> MNLEVLCGRINVENGLSLGEPGLYDQIYDRPGLPDLDVTVDATGVTVDIGAVPDSASQLGSSINAGLITIQLSEAYKINHDFTFSGLSKTTDRRLSEVFPITHDGSDGMTPAVIHTRLDGTIVVVEFSTTRSHNIGGLEAAYRTKIEKYRDPISRRVDIMENPRVFFGVIVVSSGGVLSNMPLTQDEAEELMYRFCIANEIYTKARSMDADIELQKSEEELEAISRALSFFSLFEPNIERVEGTFPNSEIKMLEQFLSTPADVDFITKTLKAKEVEAYADLCDSHYLKPEKTIQERLEINRCEAIDKTQDLLAGLHARSNKQTSLNRGTVKLPPWLPKPSSESIDIKTDSGFGSLMDHGAYGELWAKCLLDVSLGNVEGVVSDPAKELDIAISDDPEKDTPKEAKITYRRFKPALSSSARQEFSLQGVEGKKWKRMAANQKKEKESHETLSPFLDVEDIGDFLTFNNLLTDSRYGDESIQRAVSILLEKASAMQDTELTHALNDSFKRNLSSNVVQWSLWVSCLAQELASALKQHCRAGEFIIKKLKFWPIYVIIKPTKSSSHIFYSLGIRKADVTRRLTGRVFSDTIDAGEWELTEFKSLKTCKLTNLVNLPCTMLNSIAFWREKLGVAPWLVRKPCSELREQVGLTFLISLEDKSKTEEIITLTRYTQMEGFVSPPMLPKPQKMLGKLDGPLRTKLQVYLLRKHLDCMVRIASQPFSLIPREGRVEWGGTFHAISGRSTNLENMVNSWYIGYYKNKEESTELNALGEMYKKIVEMEEDKPSSPEFLGWGDTDSPKKHEFSRSFLRAACSSLEREIAQRHGRQWKQNLEERVLREIGTKNILDLASMKATSNFSKDWELYSEVQTKEYHRSKLLEKMATLIEKGVMWYIDAVGQAWKAVLDDGCMRICLFKKNQHGGLREIYVMDANARLVQFGVETMARCVCELSPHETVANPRLKNSIIENHGLKSARSLG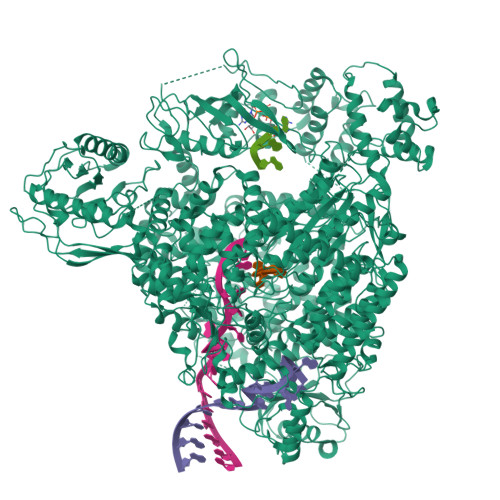PGSININSSNDAKKWNQGHYTTKLALVLCWFMPAKFHRFIWAAISMFRRKKMMVDLRFLAHLSSKSESRSSDPFREAMTDAFHGNRDVSWMDKGRTYIKTETGMMQGILHFTSSLLHSCVQSFYKSYFVSKLKEGYMGESISGVVDVIEGSDDSAIMISIRPKSDMDEVRSRFFVANLLHSVKFLNPLFGIYSSEKSTVNTVYCVEYNSEFHFHRHLVRPTLRWIAASHQISETEALASRQEDYSNLLTQCLEGGASFSLTYLIQCAQLLHHYMLLGLCLHPLFGTFMGMLISDPDPALGFFLMDNPAFAGGAGFRFNLWRACKTTDLGRKYAYYFNEIQGKTKGDEDYRALDATSGGTLSHSVMVYWGDRKKYQALLNRMGLPEDWVEQIDENPGVLYRRAANKKELLLKLAEKVHSPGVTSSLSKGHVVPRVVAAGVYLLSRHCFRFSSSIHGRGSTQKASLIKLLMMSSISAMKHGGSLNPNQERMLFPQAQEYDRVCTLLEEVEHLTGKFVVRERNIVRSRIDLFQEPVDLRCKAEDLVSEVWFGLKRTKLGPRLLKEEWDKLRASFAWLSTDPSETLRDGPFLSHVQFRNFIAHVDAKSRSVRLLGAPVKKSGGVTTISQVVRMNFFPGFSLEAEKSLDNQERLESISILKHVLFMVLNGPYTEEYKLEMIIEAFSTLVIPQPSEVIRKSRTMTLCLLSNYLSSRGGSILDQIERAQSGTLGGFSKPQKTFVRPGGGVGYKGKGVWTGVMEDTHVQILIDGDGTSNWLEEIRLSSDARLYDVIESIRRLCDDLGINNRVASAYRGHCMVRLSGFKIKPASRTDGCPVRIMERGFRIRELQNPDEVKMRVRGDILNLSVTIQEGRVMNILSYRPRDTDISESAAAYLWSNRDLFSFGKKEPSCSWICLKTLDNWAWSHASVLLANDRKTQGIDNRAMGNIFRDCLEGSLRKQGLMRSKLTEMVEKNVVPLTTQELVDILEEDIDFSDVIAVELSEGSLDIESIFDGAPILWSAEVEEFGEGVVAVSYSSKYYHLTLMDQAAITMCAIMGKEGCRGLLTEKRCMAAIREQVRPFLIFLQIPEDSISWVSDQFCDSRGLDEESTIMWG>MFKDGSLIPYLTAGDPDKQSTLNFLLALDEYAGAIELGIPFSDPIADGKTIQESHYRALKNGFKLREAFWIVKEFRRHSSTPIVLMTYYNPIYRAGVRNFLAEAKASGVNGILVVDLPVFHAKEFTEIAREEGIKTVFLAAPNTPDERLKV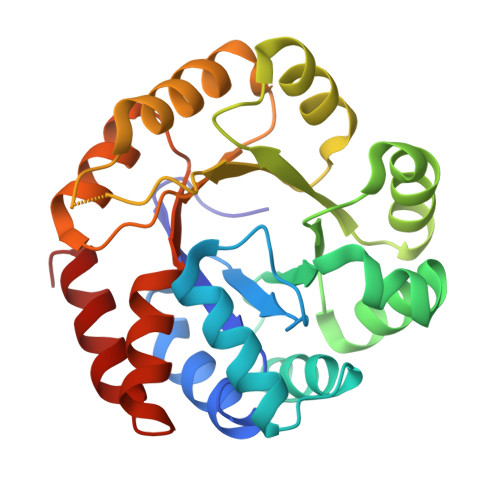IDDMTTGFVYLVSLYGTTGAREEIPKTAYDLLRRAKRICRNKVAVGFGVSKREHVVSLLKEGANGVVVGSALVKIIGEKGREATEFLKKKVEELLGI[2x]>DHHSDHQHRQHEAHVHGQVELNIAQDGHD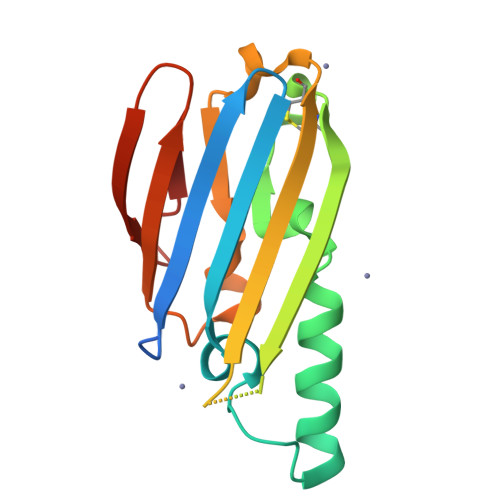LLLEITAPGADVVGFEHAPQDDAQKQALEKALETLHHPEKLFALSDKAQCEKREVLIKHTLGGEEYQHSHAYGGSFTAQYQFHCEAVDQLKQIDTQWFQYFPSTEKIQANVLTEKQQSALQLNAKQTLIKL[6x]> KRQWALEDFEIGRPLGKGKFGNVYLAREKQSKFILALKVLFKAQLEKAGVEHQLRREVEIQSHLRHPNILRLYGY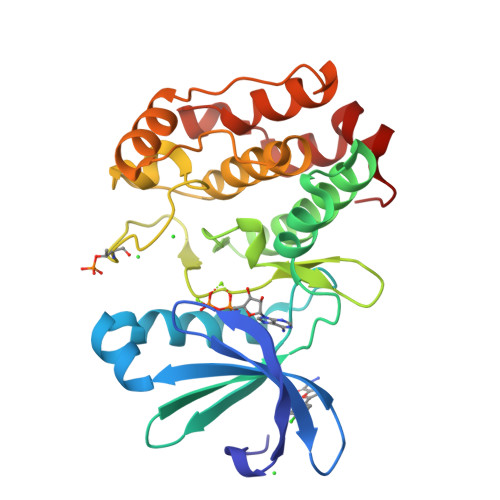FHDATRVYLILEYAPLGTVYRELQKLSKFDEQRTATYITELANALSYCHSKRVIHRDIKPENLLLGSAGELKIADFGWSVHAPSSRRTTLAGTLDYLPPEMIEGRMHDEKVDLWSLGVLCYEFLVGKPPFEANTYQETYKRISRVEFTFPDFVTEGARDLISRLLKHNPSQRPMLREVLEHPWITANSSKPS> APCKL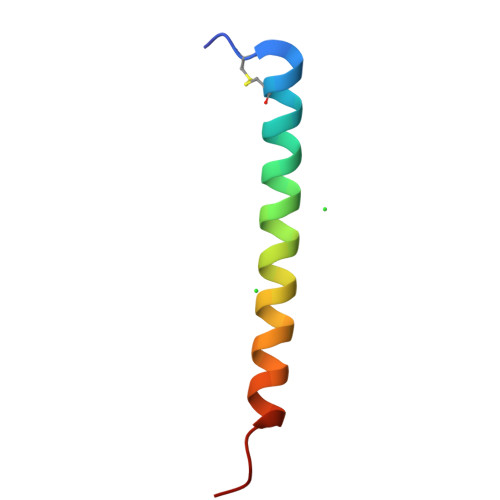GCKIKKVKQKIKQKLKAKVNAVKTVIGKISEHLG> DYKDDDDKLVPRGSCHPRLSLHRPALEDLLLGSEANLTCTLTGLRDASGVTFTWTPSSGKSAVQGPPERDLCGCYSVSSVLPGCAEPWNHGKTFTCTAAYPESKTPLTATLSKSGNTFRPEVHLLPPPSEELALNELVTLTCLARGFSPKDVLVRWLQGSQELPREKYLTWASRQEPSQGTTTFAVTSILRVAAEDWKKGD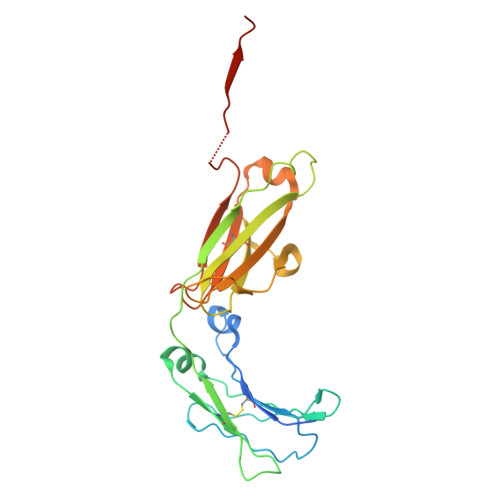TFSCMVGHEALPLAFTQKTIDRLAGKPTHVNVSVVMAEVDGTCY> DVVRASRNAKVKGKFRESYLSPAQSVKPKINTEEKLPREKLNPPTPSIYLESKRDAFSPVLLQFCTDPRNPITVIRGL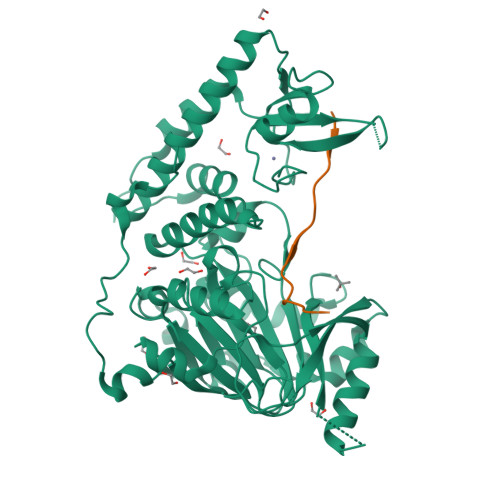AGSLRLNLGLFSTKTLVEASGEHTVEVRTQVQQPSDENWDLTGTRQIWPCESSRSHTTIAKYAQYQASSFQESLQEEKESEDEESEEPDSTTGTPPSSAPDPKNHHIIKFGTNIDLSDAKRWKPQLQELLKLPAFMRVTSTGNMLSHVGHTILGMNTVQLYMKVPGSRTPGHQENNNFCSVNINIGPGDCEWFAVHEHYWETISAFCDRHGVDYLTGSWWPILDDLYASNIPVYRFVQRPGDLVWINAGTVHWVQATGWCNNIAWNVGPLTAYQYQLALERYEWNEVKNVKSIVPMIHVSWNVARTVKISDPDLFKMIKFCLLQSMKHCQVQRESLVRAGKKIAYQGRVKDEPAYYCNECDVEVFNILFVTSENGSRNTYLVHCEGCARRRSAGLQGVVVLEQYRTEELAQAYDAFTLAPASTSRHHHHHH;> RKQLMTKAARKSAPATG4'-fluoro-4,5-dihydroxy-N-{[(1R,2R)-2-{(2S,4R,5R)-4-hydroxy-5-[6-(methylamino)-9H-purin-9-yl]oxolan-2-yl}cyclopropyl]methyl}[1,1'-biphenyl]-3-carboxamide | C27 H27 F N6 O5 | 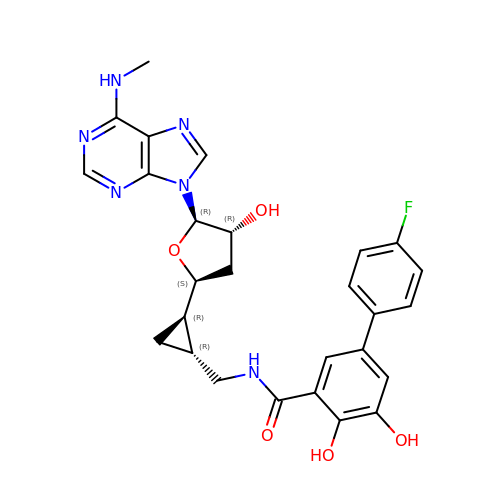HZZZGURCIAIEDZ-YJFPSUCWSA-N> MHHHHHHMPIIEQVRAREILDSRGNPTVEVEVALIDGTFARAAVPSGASTGEHEAVELRDGGDRYGGKGVQKAVQAVLDEIGPAVIGLNADDQRLVDQALVDLDGTPDKSRLGGNAILGVSLAVAKAAADSAELPLFRYVGGPNAHILPVPMMNILNGGAHADTAVDIQEFMVAPIGAPSFVEALRWGAEVYHALKSVLKKEGLSTGLGDEGGFAPDVAGTTAALDLISRAIESAGLRPGADVALALDAAATEFFTDGTGYVFEGTTRTADQMTEFYAGLLGAYPLVSIEDPLSEDDWDGWAALTASIGDRVQIVGDDIFVTNPERLEEGIERGVANALLVKVNQIGTLTETLDAVTLAHHGGYRTMISHRSGETEDTMIADLAVAIGSGQIKTGAPARSERVAKYNQLLRIEEALGDAARYAGDLAFPRFACETK

Enolase, a ubiquitous enzyme, catalyzes the reversible conversion of 2-phospho­glycerate (2PG) to phospho­enolpyruvate (PEP) in the glycolytic pathway of organisms of all three domains of life. Here we present structural snapshots of Mycobacterium tuberculosis (Mtb) enolase in apo, PEP-bound and two 2PG-bound forms as it catalyzes the conversion of PEP to 2PG. MtEno has a topology similar to other enolase structures, a smaller N-terminal domain and a larger C-terminal domain. The crystal and the cryoEM structures (enzyme in solution, frozen) along with the biochemical studies clearly demonstrate that the functional unit of MtEno is an octamer.

Of the two structures of MtEno-2PG, one harbored the widely reported 2PG-canonical pose whereas the other revealed 2PG in a novel binding pose [which we refer to as the alternate conformation (2PG-alternate)] in a manner that makes the otherwise unfavorable dissociation of the product from the active site thermodynamically feasible. Notably, 2PG in this alternate conformation has fewer hydrogen-bonding interactions in the active site due to the absence of catalytic MgB 2+. Additionally, NZ of Lys386, which interacts with O2 of 2PG only in the 2PG-canonical pose does not form any interaction in alternate-2PG. We speculate that, by switching to this alternate conformation, 2PG facilitates its dissociation from the active site by weakening the loop 1 interaction (Ser42) with 2PG on its formation from PEP. However, the MtEno–2PG-alternate exhibits a positive binding free energy of 5.5 kcal mol−1, making it thermodynamically unfavorable for the 2PG-alternate to remain bound to the active site. The higher fluctuation in the loop 1 region is largely due to the absence of MgB in the active site, and we hypothesize that the change in 2PG from the canonical to the alternate conformation deforms the MgB coordination, facilitating its release from the active site pocket. Although the crystal structures of both the MtEno–2PG exhibited closed loops, 2PG-alternate had a significantly lower number of interactions at the active site. Taken together, our study suggests that 2PG-canonical switches to 2PG-alternate in order to dissociate and exit from the active site during reverse catalysis.> MGDHSQKDSPEDFIINRLSQALGIQKEKIKKSLETQQDDKGEVTNKDEFQGFIQQDNSTNILWVSGQSEKCTFYYGQLPPIDKFKKKGIAVIKLGLHKLTNENVAKDVVVVEITNNLLEHLNSVFNEIMSPVMQNPLNQQGWTDLVAKDLMEKFNNYVAQVYVLLGQIKGKTMLPLPSHKLTSSDTTPDKDKAHVFEGSIITWTKQIKNVLKLEPEQLLKYGNDPGPLAEIEFWQNKRDNLNLIDSQLKSVEVQNILHFLDNNKSTYTTPFTKLQAEVKKARLEANENYRYLFTLKDLFSKLQESQPSDFPTLYELFIPIMHTILLIYNKSKTYNQPPRLVVLIREICNAIISNAQAFVDKDTIFSLIDSKETTEACDKLQVTLDVCSKFKDAYFEYKAKAGGNWKLTSNALFVRLDSFLERCQDILHLTNTIVQFNKLEKIELGGTKGKTLTESIAQIFKEFEEAVQAFTSVSYDIMNIAEKKFDDDFYEFRSKIKELERRLASVITQGFDDYDTIYGRFKLLDNFEGLLTRPIIADELEKKHIVLLEMYKQDLKQVQSIFLEGKQFVDSMHENAPLFLNMPPIAGALTWCKSLRDRIQEPIEKLAQLGQGITEREEYKDVQKLYTSITKSIKDYEDQKILSWEKEVEDSSQDKLKQTLLCKDENDLIKVNFDPSLVRLLKEVKYFLLLRLEVPTTAKDIYTKAETYRTQIVALDMIVDNYNHIKTCLLPVEEPLVKKKIQDMEEEVKPGIEEIRWKSTNIDQFISKSKSIVDQLFETVNKMKDSLQKIHKSLANFNVKIIERKNRPMSPDDYDQFLKAIFSNKLTIVKDNGNQIQKLVKEVLDAVKADKKQNSWKNYNDYVNVIVIEGISTAIQTALLHLNEQINPVFIKRNDISPLFDIRLELGQSGIQFDPEIGESSNQLTVRNTIRNWINDFFNIAGTIQRLDTTMPGDFLQEIRSFFEIKQCLAMITQNLEWIENECNQFRARFDTYSYLWTEDEQISFNRFLDENEPKDEDGKGGDDDEGENTEKQNPLLKGCRAKIPNLDLFDEKITHLKAIQQEISRIKTPEDISWLRINLQPMKTALDARVTRWIRVYTDFLVNQFRTTQKNLLDFIEKTKDGIKKNPADHENLHDKKLLMSVMKVISDVKDVEPRREGIITRMKEMVTKLKKHNVPITEKGTDDPLQQIDNANSNFIEIYGRVFKVKADIIPLQAEETQNIKRDLDIFMKEVESFRKEFMQKLPFDYTESMGYENINNAYDTIMVYYHKLTAIEGRALEYNNLEKLFELQKSNYKQLKDCMNDLKNLKTMWDAIALIHFQYNDWKTKPWRQIKADILLDTNKTLGTQIKNLPKEIRNFKGYNVIVEKVKNMGTVLPLVSALHSEFMEDRHWSQLKQITGTVFDHNSLSFYFEDILALNLYKYENTVNEIVDVAQKEAKIEKKLKNIEQWWSKQVFEFTEYKETKTFASLDNMMEVLDQ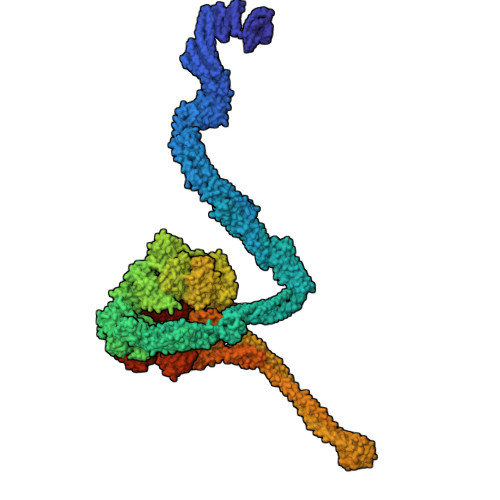HSLDLMGMKSQGKYVEFFYDRVEDWREKLGRVDVVVNEWLKVQKNWKILYNIFLLSEDIRMQLPEDTKVFEGVDKEFKDMMSEVSANPSVVEACTIERRDVLVGWSQAIKKCEKALNDYLEQKKKSFPRFYFLSNQSLLTILSNGQNAPKVCEYLGDCFDGLKTLTFEPPANPAETSKVGIGMISKDDEKVPFSSKFICEGAVEHWLLNLEFRMRETLQEILEGAKNTADLWDSGDKPREEWVEGYNAQIALLTTTIVWTEDVGRAFEDLAGGSETAMKECQKLIEVRLENLIKKVRGDLHILERWKIINIITIDVHSRDVVEKFVIQKVSEAESFAWLSQLKFYWENKPDSDMHLRQTLRFPWEKDKNKNKCIIRIVDWFRFYSYEYIGNAIRLVITPLTDRCYITLTQALNLTMGGAPAGPAGTGKTETTKDLGRAIGIPVMVFNCSDQMNKDSMAQIFMGLSQSGAWGCFDEFNRISIEVLSVVSTQVKCVLDALKEKKTKFSFVEEGEIQLQDTVGFFITMNPGYAGRTELPENLKALFRSCAMVVPDLALICENMLMSEGFTMARVLSRKFVSLYMLSRELLSKQKHYDWGLRAVKSVLRQAGKLKRGDPDMPEDPLLMRALRDFNMPKIVTDDKVIFRRLIGDLFPKLDPPTKQNPELKKIVQDTTKKDMGLVAEELFVTKVVQLAEILEVRHCCFVIGPPGSGKTCVWKTLIKSYINSGEDAEYDTLNPKAVTSDELFGAYTKTKEWKNGVIAVIMKNQVKNEEKYKATHMHKWSVLDGDIDPEWIESLNTVMDDNKVLTLVSNDRIFLTPQMRLIFEISNLRNATPATVSRAGVLFINETDIGWMPYMNSWLERSQINILKQQKEMANMPEYPVIDDVAKSVFYRCFQSYFEQNIDVHDKNRVRHICPMVDIAMIQTICTILDALLIQHLPKLKQMKEEDEKQALEAFFIFAGLWAIGGPVGGGQDDSKDMKEFNTVWKGAAKVKFPEQGLCYDYYYDINENKWNTWKVEDYLPNDQPLFSKIYVATIHTTRLRYMIDIHLQRRKPILFIGSAGTGKTAVVRDYLNSTRPEQVSHKTINFSSFTDSLALQKNIESMVEKKNGRNYGSATNKVLICFIDDFNMPYVDKYGTQSPIQLLRLILDYGSIFNREQLEERKFLQDLLFFGCLNQKSGSFTVDLRLQRNFSVFSMYTPSSDVIKTIFGSILNAHLSTIDDKAQKMAFKLVEATYFTFDKILKNTTAFAPSAKRFHYQFNFRELARVCEGICRTTPGQYSGGDQGKLVRLWAHEMKRTFEDRFIANEHVEFFRRYLTEAISKCIGEFPETENPIAEPLIFTGFVAAHQGLDQQYTQCTIPVLKRVLDDKLEEYNEVKAQMNLVLFQQAMEHVSRICRILDMPGNNALLVGVGGSGKQSLCRLSTFINGFEIDQLVVTASFTINDLRNNLQEIYKKIAKPNSIARVFMITDSQIKEEQFLIPINDMLNSGWIFDLFPKEDMDSLVSGVRNEAKGEGVDVNNLTALTSYFLDKIRKNLKVVLCFSPVGDTMRIRSRKFPGIINNTSIDWFHPWPHEALIDVAFRFLEEIEFPTEEIRQSISLNMAKVHSSIDTANEKFLKLERRYNYTTPKSFLELIDFYKKLLTEKRETIQRQIQRYEMGLNILAETQNKVQGLQEELKVKMVEVNKQREETDILIEKVGKESALAEEEQTIANAEEEKTNVAAAEAEKISKEATEALAEALPALRSAEAAVDCLKKPHVTEMKNLGSPPAGVIVTARVVLILFNQGITLNDPDEKVWKKAVTFMNNPQAFIDKVKSFDGENIEPNIIEQSNKIIQDPSKKFNEKDMAGQSYAASKLCAWAVNIVTFNKIFKQVKPLQDAQKQANEILEEKKKELAIVKQRVAELNARVNSLKRQLEEAEARKMIVEQDAARCQSRLSAAENLVNGLAGENKRWTQNVKFLKENIKSMIGDSLLASAFVSYIGAFSAKLRLELWKNTWLPDIIEKGIPITEGIEPLKILTTEAIKSKWKNEGLPADPMSLENAAIITACARWPLIIDPQLQGSTWIRGKQGENLTTISLSQPKWLGALTSSISSGRAVLIEGIQQEIDATLDPLLQRAVKKNGNQLQLEIGGDPIDYDPNFKLFLMTKLINPHFRPEIAAQCTIINFIVTESGLEEQFIAMVVNIEKNELEMAKQDLVKKQNEYAVTLDKLESDLLQSLSEADPATILDNTELIQNLDKTKKTTIEITEQQQKAKVTEAEINIQREHYRVVAAEGSMLYFLVISLSVMDHMYQYSLESFITFFFKAINRTTVRDENRIPTLILNIRQTIYQWISRGLFEKHKLIFLTLIVFRLMQKKIIDVAYEVAEMDFLIKCPARPGVENTLDWLPNISWDQIQGLINLEEFRNFAHQLEKEAPNRFKDWYNELQPEDQKLPLDWKRLDSMPFKKLLVLRCLRPDRMTISLNNFIRAVLPQGDAFVEMDQKLAFSEILESVINEDSESTIPIFFILSPGSDPVKEVEKIAKKKRIEPGKNFFNIALGQGQDEIARRRIEEGNKEGHWVMLQNIHLMPTWLIELEKILDSYSGEAGGGNSEFRLFLSAEPSTGIPIGILDRSIKLTNEPPAGLKANMKRAWTYFSKEEIEDKDPKIKSILFALCFFHSTLIERRRFGPKGWNMSYPFNMGDLRDSYLVMNRYMEQNQGGKVPFNDLIYIFGEIMYGGHIVDDWDRRLCNSYLFNTMHEQLFDELELFPYIEGKGLSFKVPGQNPYEKYIEHIETSLKQETPLAYGLHPNAEIGFRTDQCKTLFNTLLELMPKEQSRDEKSSDIKSSNEMASDLIKQLLEDSELKNKIFNMEEIKNKIDAENKGPYQNVFLQEIEYMNALLSEIVKDLEEIGQGLSGLLTVSENMEMIIESIALSRVPASWQKLAYPSKRGLQSWLANLFQRIEQLNIFRDDPYSIPRVVMISRFFNPQSFLTAIMQVISRAKAYELNKLYIQTEITKRSIEEIEGAAKEGAYVYGFILEGARWDYQLGQLEESKPKEMFSVLPVTYCKAIPLPPEGKEDKSLYQCPVYKTEDRGNTYVFTAQLKTRFPPRKWILAGVAIIMDVEGVSD Diploptera punctata, also known as the Pacific beetle cockroach, is a viviparous cockroach that gives birth to live offspring and secretes a highly concentrated mixture of glycosylated proteins as a source of nourishment for developing embryos. The principal component of this milk is lipocalin-like proteins or Lili-Mips. Lili-Mip has a lipocalin fold and binds to different fatty acids and other moieties. Lili-Mip is small (18.8 kDa), monomeric, and glycosylated.

The structure of Lili-Mip2 showed that in the ligand-binding pocket, Glu-38 is held in position by hydrogen bonds from His-115 and Tyr-40, enabling ligand binding. We hypothesized that the kink formed by E38 in Lili-Mips results in a preference for the binding of unsaturated fatty acids, with the unsaturated bond occupying the position at the kink. The mutation of Glu-38 to alanine was predicted to influence ligand binding. Mutation to alanine only slightly altered the positions of Tyr-40 and His-115. Mass spectrometry analysis showed that all Lili-Mip isoforms (and Lili-Mip2-E38A) bound abundantly to palmitoleic acid (16:1), palmitic acid (16:0), oleic acid (18:1), and stearic acid (18:0). Lili-Mip2-E38A did not exhibit fluorescence intensity change on ligand binding. Therefore, we could not measure ligand binding affinity even though mass spectrometry analysis showed fatty acid binding. The crystal structure of Lili-Mip2-E38A suggested that the binding cavity did not extend to tryptophan. In the bound fatty acid in the structure, the distance between the terminal methyl group of the acyl chain of the fatty acid and the ring of the Trp is 8.4 Å, compared to 3.8 Å in Lili-Mip 2. We propose that binding of the fatty acid at that distance will not significantly change the tryptophan environment resulting in a change in intrinsic tryptophan fluorescence.

> KEPCPPENLQLTPRALVGKWYLRTTSPDIFKQVSNITAFYSAHGNDYYGTVTDYSPEYGLEAHRVNLTVSGRTLKFYMNDTHEYDSEYEILAVDKDYFIFYGHPPAAPSGLALIHYRQSCPKEDIIKRVKKSLKNVCLDYKYFGNDTSVHCRYLE> GAMAPPFFDLKPVSVDLALGESGTFKCHV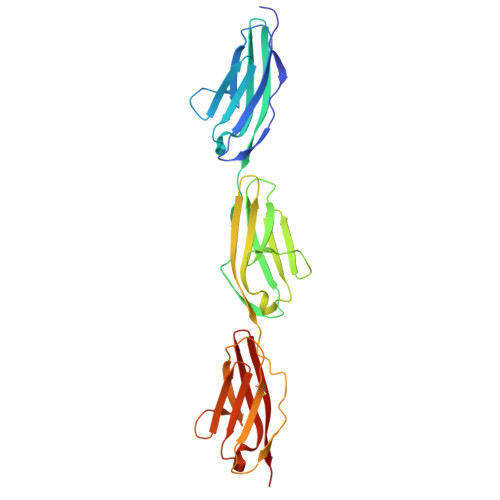TGTAPIKITWAKDNREIRPGGNYKMTLVENTATLTVLKVTKGDAGQYTCYASNVAGKDSCSAQLGVQAPPRFIKKLEPSRIVKQDEHTRYECKIGGSPEIKVLWYKDETEIQESSKFRMSFVESVAVLEMYNLSVEDSGDYTCEAHNAAGSASSSTSLKVKEPPVFRKKPHPVETLKGADVHLECELQGTPPFQVSWHKDKRELRSGKKYKIMSENFLTSIHILNVDSADIGEYQCKASNDVGSYTCVGSITLKA> LEEHYYSRKTCGSGGGLSVQRTGYPQTDPPVFKAVNSFERAPLIVGDHVHSLPYWSRKITLECTPYPFTLRWEGGVHKDGIPDKVPHPSCDPGSELVSYTHSREVDCERFIGPVPSSFTDPKVTSAQWKFLEDMADMKA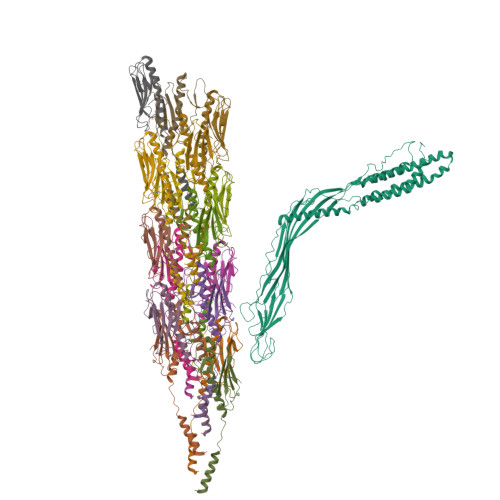LADLNKSLVNLPMLYKERRETLKMVGNRLGGLVRVAHAAQDRDLKRYFKARRKDRRKVAEEVANGHLELIFGWLPLIGELEGAIEYAELPDLDFIRCHGLHTLVLQSTPWDNSVDVRSYPNWERAAGTRITGSVRTRGVVESRASVRTALRFNLETSLAGDARRLGFEPISTTYDMIPLSFVVGWFSNFDKYVRTLAPLIGVTFETGSQNRRTTCELVGCTRFYPRTVSPPSGWFARWKDFPDGSLSEVSGLRRTDIRSVLSTLPDPDVRFHADVGLFEISAGISLLAQRYLKPLQRLLKRKSFFYGRT;>FTLIELMIVVAIIGILAAIAIPQYQNYVARSEGASALATINPLKTTVEESLSRGIAGSKIKIGTTASTATETYVGVEPDANKLGVIAVAIEDSGAGDITFTFQTGTSSPKNATKVITLNRTADGVWACKSTQDPMFTPKGCDN[16x]>[12x]MTGNDVQGAEKADAIGMVLGTEDVTPTVFWFAVSHGASVGLDDLVVVETRKPDGTPVRFYGLVDNVRKRHEGVTFESDVEDVVAGLLPASVSYAARVLVTRVDPENFIPPQPGDHVRHAAGRELAMALSADKMEEAAFPGGLLADGQPLPLNFRFINGESGGHINISGISGVATKTSYALFLLHSIFRSGVMDRTAQGSGGRQSGTAGGRALIFNVKGEDLLFLDKPNARMVEKEDKVVRAKGLSADRYALLGLPAEPFRDVQLLAPPRAGAAGTAIVPQTDQRSEGVTPFVFTIREFCARRMLPYVFSDASASLNLGFVIGNIEEKLFRLAAAQTGKGTGLIVHDWQFEDSETPPENLDFSELGGVNLQTFEQLISYLEYKLLEEREGEGDPKWVLKQSPGTLRAFTRRLRGVQKYLSPLIRGDLTPEQAEGYRPDPLRRGIQLTVVDIHALSAHAQMFVVGVLLREVFEYKERVGRQDTVFVVLDELNKYAPREGDSPIKDVLLDIAERGRSLGIILIGAQQTASEVERRIVSNAAIRVVGRLDLAEAERPEYRFLPQSFRGRAGILQPGTMLVSQPDVPNPVLVNYPFPAWATRRDEVDDLGGKAAAEVGAGLLR

The nuclease NurA and the ATPase/translocase HerA play a vital role in repair of double-strand breaks (DSB) during the homologous recombination in archaea. HerA is a circular ATP-dependent bipolar translocase and helicase; it belongs to the HerA/FtsK bacterial translocases family, an offshoot of the RecA family. Each drHerA protomer comprises three domains: the N-terminal HerA-ATP synthase barrel domain (HAS-barrel domain) that forms the putative exit for the substrate, the RecA-like ATPase domain, and the helix-bundle domain which is inserted into the RecA-like ATPase domain and forms the putative entrance for the substrate. Herein, we characterized, for the first time, the crystal structures of D. radiodurans HerA (drHerA), with and without ADP binding, and a low-resolution cryo-EM structure of the drNurA-HerA complex.

The drHerA-ADP complex was crystallized in space group P212121, and the structure was solved at 3.4 Å resolution by the molecular replacement method using drHerA apo structure as the search model. The refined drHerA-ADP complex model contains two hexamers (twelve protomers) in the asymmetric unit; each protomer is bound to one ADP molecule. Although ADP•AlF3 was used as an ATP analog for crystallization, the density of aluminum fluoride, which represents the γ-phosphate position in the transition state, is missing in the density map. The residue Lys217 and the trans-acting residue Arg513, as well as Arg154 in the neighboring subunit, which is supposed to bind the γ-phosphate group of ATP molecule, are located quite far away from the ligand in this structure. Therefore, this ligand-binding structure was considered as a drHerA-ADP complex. The binding of ADP resulted in each RecA-like domain to move closer to the neighboring RecA-like domain, generating a more tightened hexamer but still a more-or-less flat ring. The overall structure of drHerA-ADP has a height of 100 Å and its outside diameter is approximately 105 Å. Interestingly, the hexamer displays a certain asymmetry, with ~26–28.5 Å inside diameter of the putative DNA translocation motifs, ~23–25.5 Å inside diameter of the putative DNA entrance, and ~27.5–29 Å inside diameter of the putative DNA exit. Such asymmetry is probably due to the differences of ADP-binding states or simply because of crystal packing. In this motif, the conserved lysine (K175) forms ion pairs with the β-phosphate and the threonine residue (T176) coordinates a Mg2+ ion.>[4x]GHMQ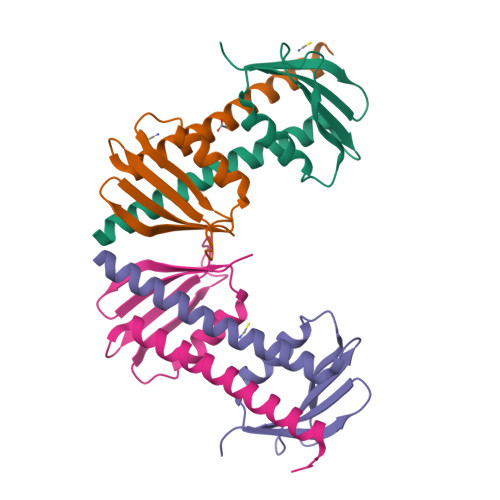RERTAESSLRVISKEKNSITVEMINYDNTLLRTLVEEILKDDQVDEARYYIKHPVIDNPQIYVRVKSGKPQSAIKRAVRKLSKLYEDLGTQFQKEFQRYESDHMIKAVEGS> DNQFYSVEVGDSTFTVLKRYQNLKPIGSGAQGIVCAAYDAVLDRN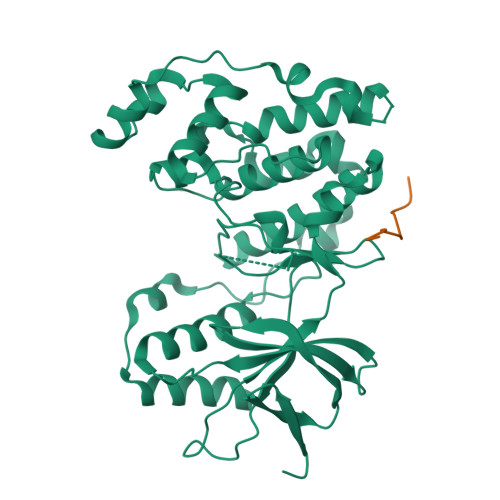VAIKKLSRPFQNQTHAKRAYRELVLMKCVNHKNIISLLNVFTPQKTLEEFQDVYLVMELMDANLCQVIQMELDHERMSYLLYQMLCGIKHLHSAGIIHRDLKPSNIVVKSDCTLKILDFGLARTAGTSFMMTPYVVTRYYRAPEVILGMGYKENVDIWSVGCIMGEMVRHKILFPGRDYIDQWNKVIEQLGTPCPEFMKKLQPTVRNYVENRPKYAGLTFPKLFPDSLFPADSEHNKLKASQARDLLSKMLVIDPAKRISVDDALQHPYINVWYDPAEVEAPPPQIYDKQLDEREHTIEEWKELIYKEVMN;> PKRPTTLNLF>MSNLLTVHQNLPALPVDATSDEVRKNLMDMFRDRQAFSEHTWKMLLSVCRSWAAWCKLNNRKWFPAEPEDVRDYLLYLQARGLAVKTIQQHLGQLNMLHRRSGLPRPSDSNAVSLVMRRIRKENVDAGERAKQALAFERTDFDQVRSLMENSDRCQDIRNLAFLGIAYNTLLRIAEIARIRVKDISRTDGGRMLIHIGRTKTLVSTAGVEKALSLGVTKLVERWISVSGVADDPNNYLFCRVRKNGVAAPSATSQLSTRALEGIFEATHRLIYGAKDDSGQRYLAWSGHSARVGAARDMARAGVSIPEIMQAGGWTNVNIVMNYIRNLDSETGAM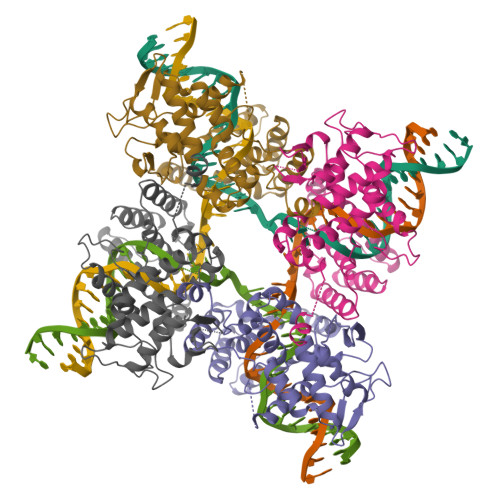VRLLEDGD[2x]> MQRFIRHSMRQIAVLGLLAGMMASVQAGADHRLDDITARGVLRVGTTGDYKPFSSRAGNDFVGLDIELAADLARTLGVPVQIVPTSWPTLMKDFGDGKFDIALGGVSITPERQKQGLFSVSYLRDGKTPITRCENSARFQ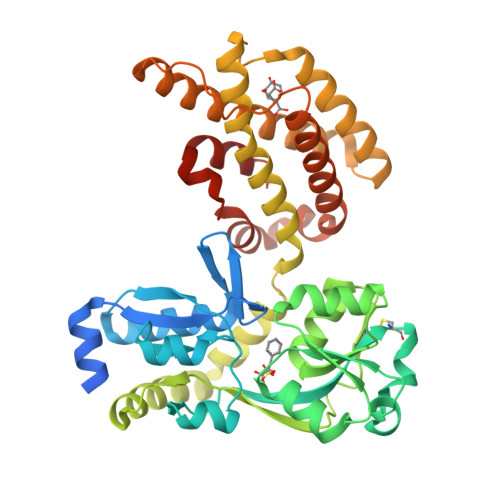TLAQIDQPGVRLVVNPGGTNERFARSQAPNAQLTVYPDNVTIFDQIVTGAADLMITDAIETRLQQRLRPQLCAVHPDTPFDFAEKAILLPRDVAFKAVVDKWLQQRIASGAVQRSVDRWLDFPWGLEPLRLAIDQRLLLAQAVARAKWNVQAPIEDLGREAQVIQAAVKEGAALGLPKVWIETVFRAQIEASKTVQRELFAQWSAQQAGKFDDAPDLAKTIRPELDRLTTQLLRSMASNQTVLNDEARKADVARAMRALEARALSPQAATQALAPFFLEHHHHHH> GMANKVEHRLSEQQMKALTDLPLVFLITHDQSKSWPITHAISWVYAKDETTIRFAIEADSLLVKTLADHPVFTLIFFADQSTYSLTCTDVAAW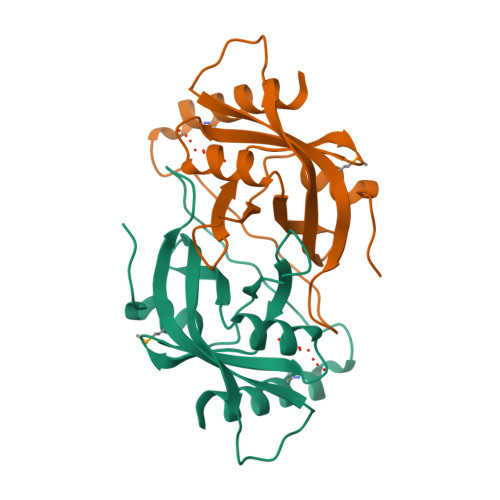ETTARLPLKVALYEGQIKEVRDILFYGAAVSDRPRVYKTYDEAAAMQLDQQIQDILKG> WSAQDKHKEGVNSHLWIVNRAIDIMSRNTTLVKQDRVAQLNEWRTELENGIYAADYENPYYDNSTFASHFYDPDNGKTYIPFAKQAKETGAKYFKLAGESYKNKDMKQAFFYLGLSLHYLGDVNQPMHAANFTNLSYPQGFHSKYENFVDTIKDNYKVTDGNGYWNWKGTNPEEWIHGAAVVAKQDYSGIVNDNTKDWFVKAAVSQ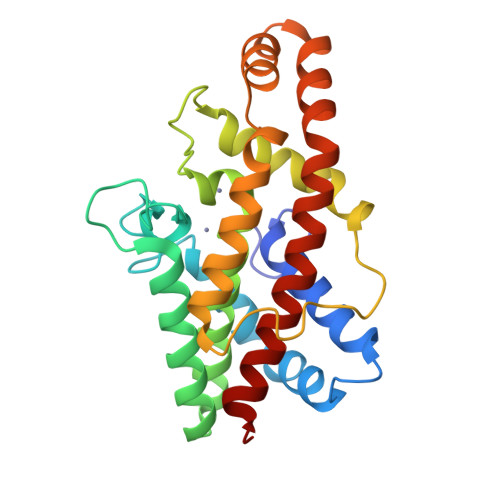EYADKWRAEVTPMTGKRLMDAQRVTAGYIQLWFDTYGDR>GSHMGDLKYSLERLREILERLEENPSEKQIVEAIRAIVENNAQIVEAIRAIVENNAQIVENNRAIIEALEAIGGHNKILEEMKKQLKDLKRSLERG[3x]

We used de novo protein design to generate very closely related proteins that adopt two very different states—a short state and a long state, like a viral fusion protein—and then created a single molecule that can be found in both forms. Inspired by class I viral fusion proteins, such as influenza hemagglutinin, we chose homotrimeric helical bundles as the fundamental architecture. We decided on a design scheme with two divergent conformations containing a constant six-helix bundle “base” and a variable portion with three inner helices and three “flipping” helices. In the compact “short” state (∼66 Å height), the flipping helices fold back to interact with the inner helices; in the extended “long” state (∼100 Å height), they extend to form interactions with each other.

The interaction energy between the flipping helix and the inner helices in the short state was tuned by combining hydrogen bond layers (“A”) or hydrophobic layers (“X”) in different orders in each of three possible positions. Designs were given three-letter names corresponding to the layers in order, starting at the hinge proximal position. In the long state but not in the short state, the “key” hinge residue (G75) and the “backup” hinge residue (T76) have the potential to form an ion coordination site. We sought to design calcium- or nickel-binding sites in the long state by introducing aspartic acid or histidine at the key hinge residue position. Crystal structures were determined for all potential bistable candidates (XAX_GGDQ, XXA_GVDQ, XAA_GGHN, and XAA_GVDQ), and we chose to focus on XAA_GVDQ because of the presence of a bound calcium. Given that changes in three residues in the hinge region can change the conformation of the design (hinge GGHN is long; GGGT is short), future work on these residues may yield designs that populate soluble short and long states in equilibrium and are switchable in solution conditions.>[2x]WVQPITAQKPSLTLWLDDKMFTGLINTGADVTIIKLEDWPPNWPITDTLTNLRGIGQSNNPKQSSKY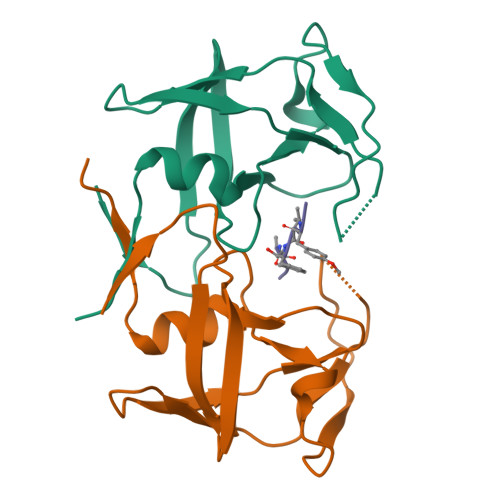LTWRDKENNSGLIKPFVIPNLPVNLWGRDLLSQMKIMMASPNDIVTA;> PYVFAMT> TDEITSFSIPKFRPDQPNLIFQGGGYTTKEKLTLTKAVKNTVGRALYSLPIHIWDSETGNVADFTT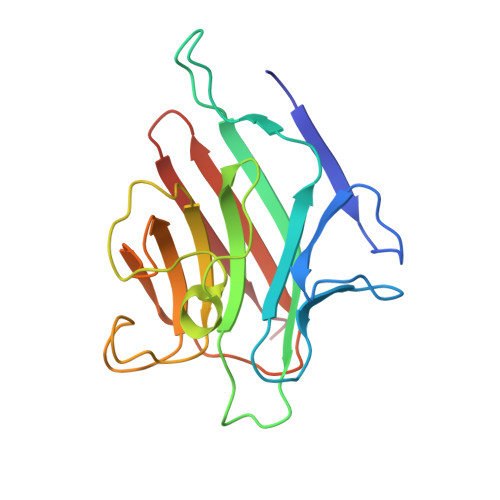TFIFVIDAPNGYNVADGFTFFIAPVDTKPQTGGGYLGVFNGKDYDKTAQTVAVEFDTFYNAAWDPSNGKRHIGIDVNTIKSISTKSWNLQNGEEAHVAISFNATTNVLSVTLLYPN> MAHHHHHHHHHHGALEVLFQGPGDPTVFHKRYLKKIRDLGEGHFGKVSLYCYDPTNDGTGEMVAVKALKADAGPQ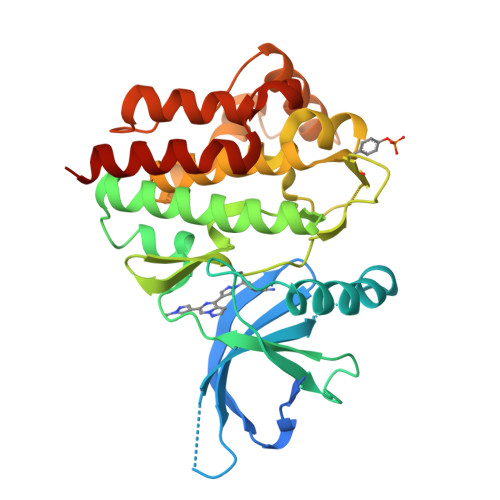HRSGWKQEIDILRTLYHEHIIKYKGCCEDAGAASLQLVMEYVPLGSLRDYLPRHSIGLAQLLLFAQQICEGMAYLHSQHYIHRDLAARNVLLDNDRLVKIGDFGLAKAVPEGHEYYRVREDGDSPVFWYAPECLKEYKFYYASDVWSFGVTLYELLTHCDSSQSPPTKFLELIGIAQGQMTVLRLTELLERGERLPRPDKCPAEVYHLMKNCWETEASFRPTFENLIPILKTVHEKYQGQAPS>MTNIQKRFYKGRVALNVLANNIENAKDIFEAAEGYVVVGVLSKDYPTVEEAVTAMKAYGKEIEDAVSIGLGAGDNRQAAVVAEIAKHYPGSHINQVFPSVGATRANLGGKDSWINSLVSPTGKVGYVNISTGPISAAGEEKAIVPIKTAIALVRDMGGNSLKYFPMKGLAHEEEYRAVAKACAEEGFALEPTGGIDKENFETIVRIALEANVERVIPHVYSSII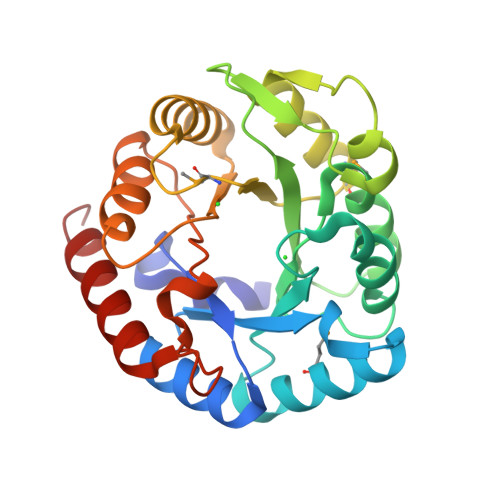DKETGNTKVEDVRELLAVVKKLVDQYA[2x]>[2x]MTEPL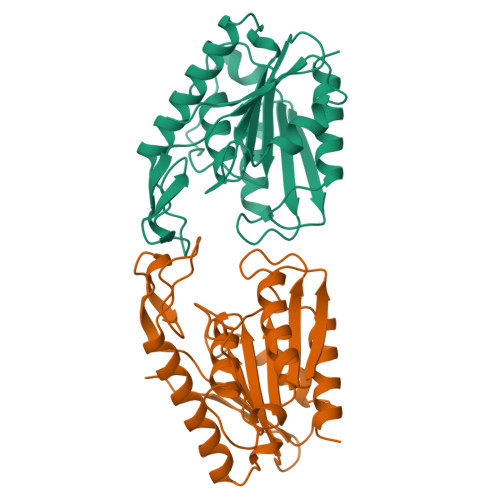ILQPAKPADACVIWLHGLGADRYDFMPVAEALQESLLTTRFVLPQAPTRPVTINGGYEMPSWYDIKAMSPARSISLEELEVSAKMVTDLIEAQKRTGIDASRIFLAGFSQGGAVVFHTAFINWQGPLGGVIALSTYAPTFGDELELSASQQRIPALCLHGQYDDVVQNAMGRSAFEHLKSRGVTVTWQEYPMGHEVLPQEIHDIGAWLAARLG> GTSHLVKCAEKEKTFCVNGGECFMVKDLSNPSRYLCKCPNEFTGDRC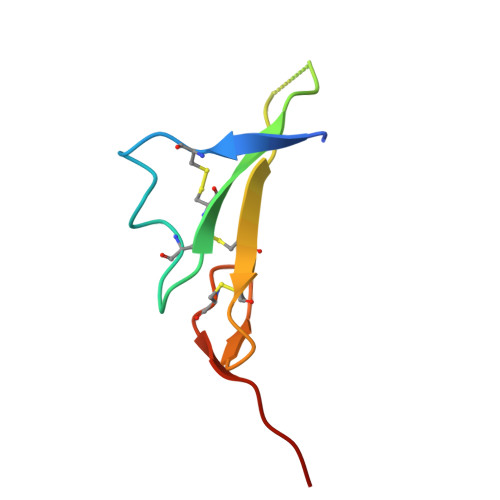QNYVMASF> MDDDDKMDNECTTKIKPRIVGGTASVRGEWPWQVTLHTTSPTQRHLCGGSIIGNQWILTAAHCFYGVESPKILRVYSGILNQSEIKEDTSFFGVQEIIIHDQYKMAESGYDIALLKLETTVGYGDSQRPICLPSKGDRNVIYTDCWVTGWGYRKLRDKIQNTLQKAKIPLVTNEECQKRYRGHKITHKMICAGYREGGKDACKGDSGGPLSCKHNEVWH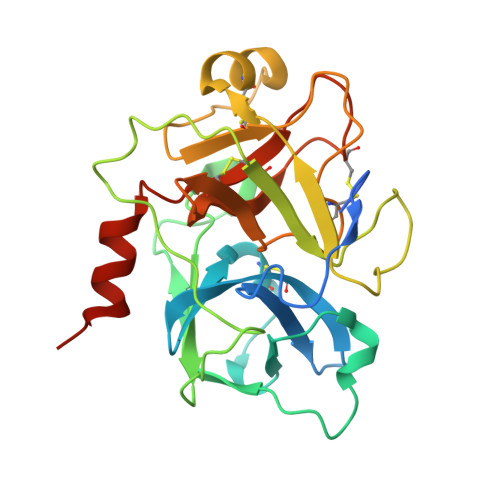LVGITSWGEGCAQRERPGVYTNVVEYVDWILEKTQAVHHHHHH> GPHMARKFFVGGNWKANGTAEEVKKIVNTLNEAQVPSQDVVEVVVSPPYVFLPLVKSTLRSDFFVAAQNCWVKKGGAFTGEVSAEMLVNLDIPWVILGHSERRAILNESSEFVGDKVAYALAQGLKVIACVGETLEEREAGSTMDVVAAQTKAIADRVTNWSNVVIAYEP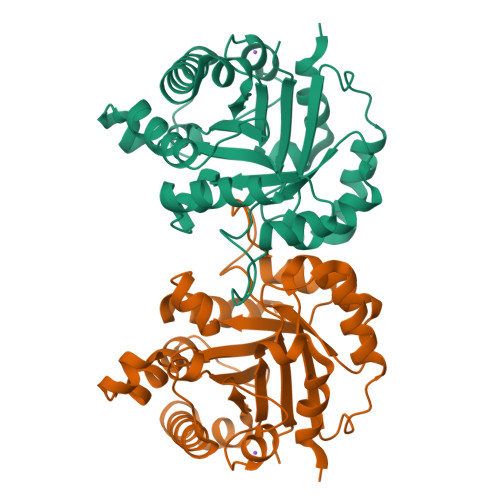VWAIGTGKVASPAQAQEVHDELRKWLAKNVSADVAATTRIIYGGSVNGGNCKELGGQADVDGFLVGGASLKPEFIDIIKAAEVKKSA>[2x]GSMVKVAILGASGGVGQPLSLLLKLSPYVSELALYDIRAAEGIGKDLSHINTNSSCVGYDKDSIENTLSNAQVVLIPAGVPRKPGLTRDDLFKMNAGIVKSLV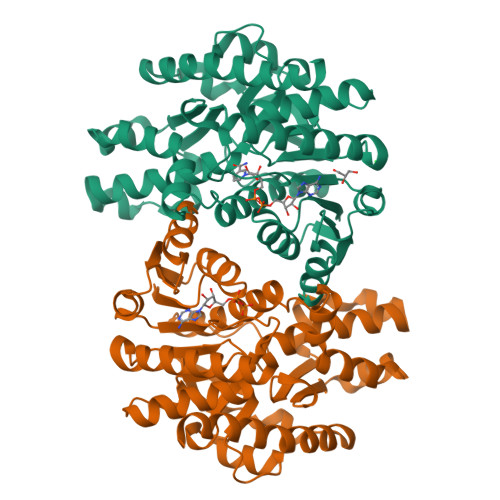TAVGKFAPNARILVISNPVNSLVPIAVETLKKMGKFKPGNVMGVTNLDLVRAETFLVDYLMLKNPKIGQEQDKTTMHRKVTVIGGHSGETIIPIITDKSLVFQLDKQYEHFIHRVQFGGDEIVKAKQGAGSATLSMAFAGAKFAEEVLRSFHNEKPETESLSAFVYLPGLKNGKKAQQLVGDNSIEYFSLPIVLRNGSVVSIDTSVLEKLSPREEQLVNTAVKELRKNIEKGKSFILDSSKL>[5x]G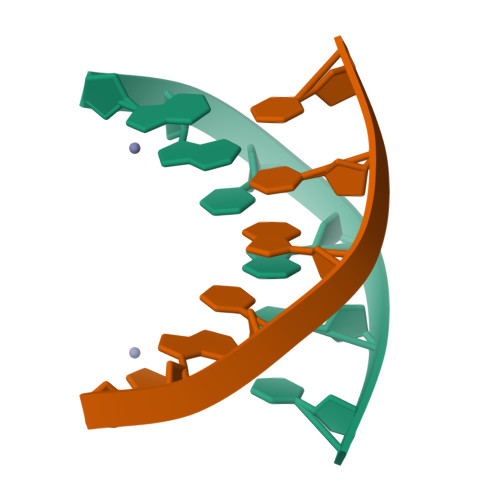GCGCC>WGQGTLVTVSAESARNPTIYPLTLPPALSSDPVIIGCLIHDYFPSGTMNVTWGKSGKDITTVNFPPALASGGRYTMSSQLTLPAVECPEGESVKCSVQHDSNPVQELDVNCSGPTPPPPITIPSCQPSLSLQRPALEDLLLGSDASITCTLNGLRNPEGAVFTWEPSTGKDAVQKKAVQNSCGCYSVSSVLPGCAERWNSGASFKCTVTHPESGTLTGTIAKVTVNTFPPQVHLLPPPSEELALNELLSLTCLVRAFNPKEVLVRWLHGNEELSPESYLVFEPLKEPGEGATTYLVTSVLRVSAETWKQGDQYSCMVGHEALPMNFTQKTIDRLSGKPTNVSVSVIMSEGDGICY[4x];> DDEATILADNKCMCTRVTSRIIPSTEDPNEDIVERNIRIVVPLNNRENISDPTSPLRRNFVYHLSDVCKKCD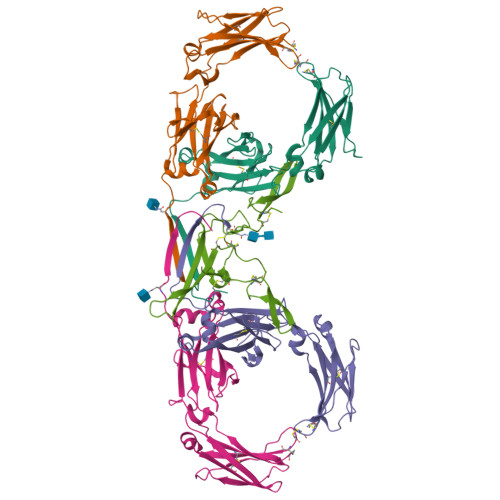PVEVELEDQVVTATQSNICNEDDGVPETCYMYDRNKCYTTMVPLRYHGETKMVQAALTPDSCYPD> MKQECNVCYFNLPDPESTLGPYDNELNYFTWGPGFEYEPEPQRKPLSIEESFENSEESEESVADIQQLEEKVDESDVRIYFNEKSSGGKISIDNASYNARKLGLAPSSIDEKKIKELYGDNLTYEQYLEYLSICVHDKDNV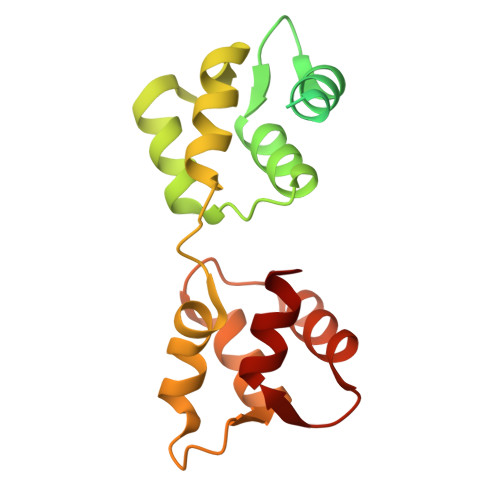EELIKMFAHFDNNCTGYLTKSQMKNILTTWGDALTDQEAIDALNAFSSEDNIDYKLFCEDILQ> MENTENSVDSKSIKNLEPKIIHGSESMDSGISLDNSYKMDYPEMGLCIIINNKNFHKSTGMTSRSGTDVDAANLRETFRNLKYEVRNKNDLTREEIVELMRDVSKEDHSKRSSFVCVLLSHGEEGIIAGTNGPVD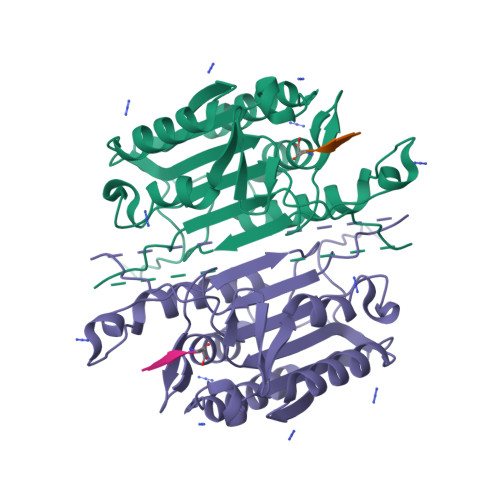LKKITNFFRGDRCRSLTGKPKLFIIQACRGTELDCGIETDSGVDDDMACHKIPVEADFLYAYSTAPGYYSWRNSKDGSWFIQSLCAMLKQYADKLEFMHILTRVNRKVATEFESFSFDATFHAKKQIPCIVSMLTKELYFYHLH> MGGGPNTGRD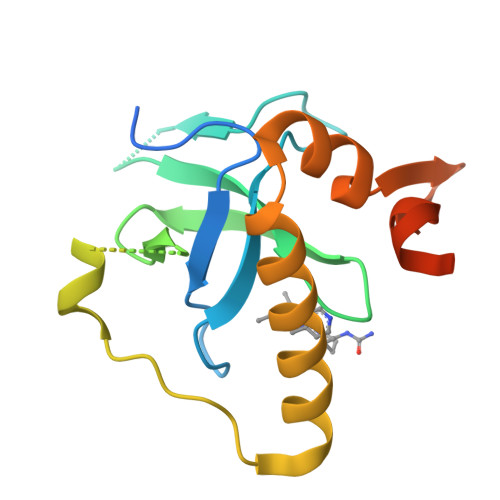KDHLLKYNVGDLVWSKVSGYPWWPCMVSADPLLHSYTKLKGQAASARQYHVQFFGDAPERAWIFEKSLVAFAGEGQFAKLCQESAKQAPTAAEKIKLLAPISGKLRAQWEMGIVQAEEAASMSVEERKAKFTFLYVGAQLHLNPQVAKEAGIAAEGGGENLYFQ>STQEQTPQICVVGSGPAGFYTAQHLLKHHSRAHVDIYEKQLVPFGLVRFGVAPDHPEVKNVINTFTQTARSDRCAFYGNVEVGRDVTVQELQDAYHAVVLSYGAEDHQALDIPGEELPGVFSARAFVGWYNGLPENRELAPDLSCDTAVILGQGNVALDVARILLTPPDHLEKTDITEAALGALRQSRVKTVWIVGRRGPLQVAFTIKELREMIQLPGTRPMLDPADFLGLQDRIKEAARPRKRLMELLLRTATEKPGVEEAARRASASRAWGLRFFRSPQQVLPSPDGRRAAGIRLAVTRLEGIGEATRAVPTGDVEDLPCGLVLSSIGYKSRPIDPSVPFDPKLGVVPNMEGRVVDVPGLYCSGWVKRGPTGVITTTMTDSFLTGQILLQDLKAGHLPSGPRPGSAFIKALLDSRGVWPVSFSDWEKLDAEEVSRGQASGKPREKLLDPQEMLRLLGH[2x];>GSSEDKITVHFINRDGETLTTKGKIGDSLLDVVVQNNLDIDGFGACEGTLACSTCHLIFEQHIFEKLEAITDEENDMLDLAYGLTDRSRLGC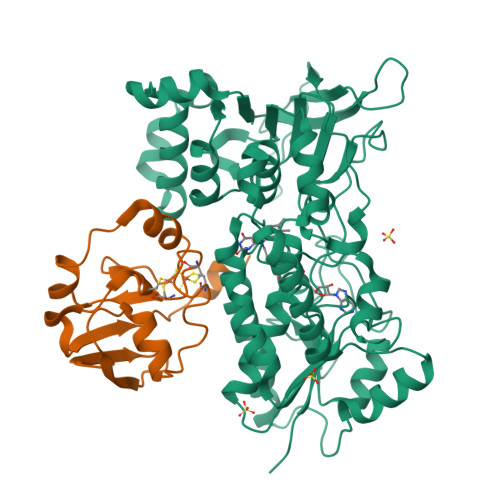QICLTKAMDNMTVRVPDAVSDARESIDMGMNSSKIE[2x]> MSKILVIAEHRRNDLRPVSLELIGAANGLKKSGEDKVVVAVIGSQADAFVPALSVNGVDELVVVKGSSIDFDPDVFEASVSALIAAHNPSVVLLPHS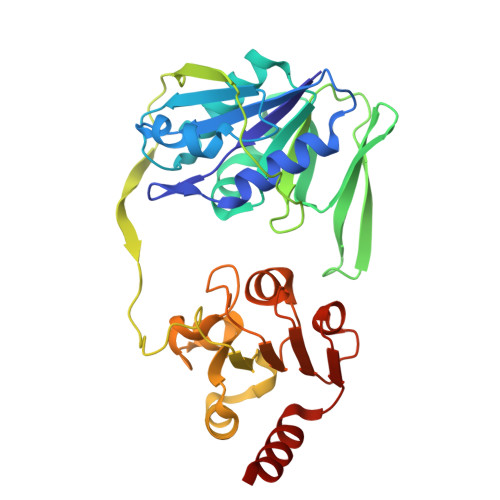VDSLGYASSLASKTGYGFATDVYIVEYQGDELVATRGGYNQKVNVEVDFPGKSTVVLTIRPSVFKPLEGAGSPVVSNVDAPSVQSRSQNKDYVEVGGGNDIDITTVDFIMSIGRGIGEETNVEQFRELADEAGATLCCSEPIADAGWLPKSRQVGQSGKVVGSCKLYVAMGISGSIQHMAGMKHVPTIIAVNTDPGASIFTIAKYGIVADIFDIEEELKAQLAA> SA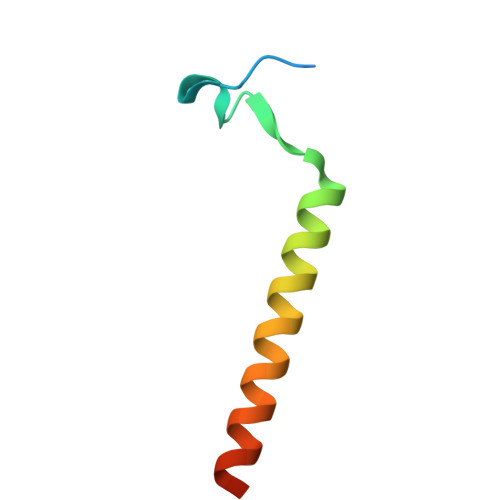CKETGWPFCSDEDWNTKCPSGCRMKGLIDEVDQDFTSRINKLRDSLFNYQK> GSSVVVDTNGQPVSNGADAYYLVPVSHG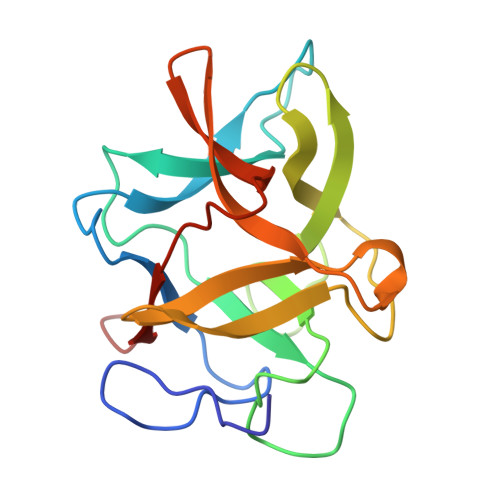HAGLALAKIGNEAEPRAVVLDPHHRPGLPVRFESPLMINIIKESYFLNIKFGPSSSDSGVWDVIQQDPIGLAVKVTDTKSLLGPFKVEKEGEGYKIVYYPERGQTGLDIGLVHRNDKYYLAVKDGEPCVFKIRKATDE>[2x]MLKNKTRAEKYQTYYTTNEYQIVKEKLPDIIRDAEIKASEVLEPTIYEKRAIMEVIKDFIRDHQRKVYGGTALNEALKQVNPKDAIYDNYSFSDIEFYSPTPVQDLVDLCNILYRKGYKFVQGKDAQHEETYSIFVNFQLYCDITYSPTRVFYGIKTIEIDGINYTDPHFMLIDYLRMVNQPLTAAGQRWEKAFERMYRLLKDYPIEDFDKRLDIPEPPEEIQSYISRIKTEFLSDNKLNESFLISGIEAYNFYIRHAASSKDEEQMARTNRNVVNLNNFIANVPFSELISVNYREDVKNTYNFLRMIVEDKEKISVDEYFPLFQFTGY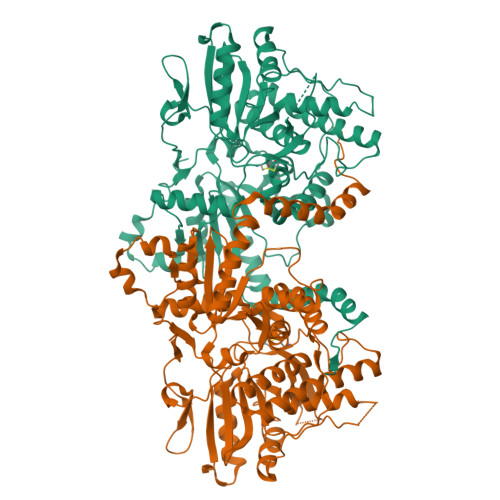STVIKYDDHPIIRIYEGDGYCIPNVKTVKTVENDNGTKTKYEYKYVSFQYVLMILYINKFRAHLDKNKPMYFNYGIAISNLVKARNIYLDQTGKSVLDNTVFKEFRTNCTGNTISFTRMNRLRLLEKRKQGKQTSFVYTPEDFFKKDLETQAKLDPSKARFKNTSGNKIMVPKYLLFKIDNNGNIEDNIHSEEAEISEKEETSGGSSISTDKSFEESPNSSPNSSPNNSLNNSIDISTNNYDDRSENSLDSLTSD>[3x]AQVINTFDGVAD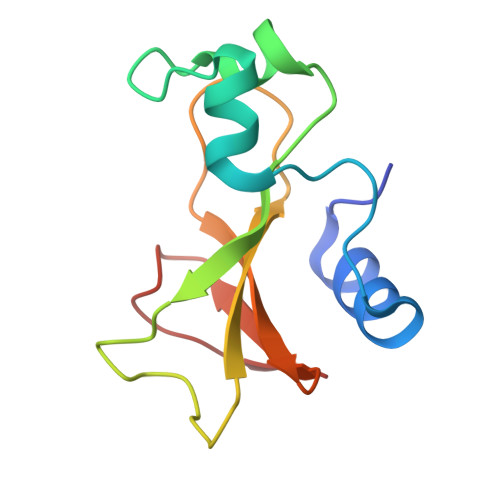YLQTYHKLPDNYITKSEAQALGWVASKGNLADVAPGKSIGGDIFSNREGKLPGKSGRTWREADVNYTSGFRNSDRILYSSDWLIYKTTDHYQTFTKIR>MTTELNQGEQFVADFRANAAALTTANAYNPEDEHDACGVGFIAAIDGKPRRSVVEKGIEALKAVWHRGAVDADGKTGDGAGIHVAVPQKFFKDHVKVIGHRAPDNKLAVGQVFLPRISLDAQEACRCIVETEILAFGYYIYGWRQVPINVDIIGEKANATRPEIEQIIVGNNKGVSDEQFELDLYIIRRRIEKAVKGEQINDFYICSLSARSIIYKGMFLAEQLTTFYPDLLDERFESDFAIYHQRYSTNTFPTWPLAQPFRMLAHNGEINTVKGNVNWMKAHETRMEHPAFGTHMQDLKPVIGVGLSDSGSLDTVFEVMVRAGRTAPMVKMMLVPQALTSSQTTPDNHKALIQYCNSVMEPWDGPAALAMTDGRWVVGGMDRNGLRPMRYTITTDGLIIGGSETGMVKIDETQVIEKGRLGPGEMIAVDLQSGKLYRDRELKDHLATLKPWDKWVQNTTHLDELVKTASLKGEPSDMDKAELRRRQQAFGLTMEDMELILHPMVEDGKEAIGSMGDDSPIAVLSDKYRGLHHFFRQNFSQVTNPPIDSLRERRVMSLKTRLGNLGNILDEDETQTRLLQLESPVLTTAEFRAMRDYMGDTAAEIDATFPVDGGPEALRDALRRIRQETEDAVRGGATHVILTDEAMGPARAAIPAILATGAVHTHLIRSNLRTFTSLNVRTAEGLDTHYFAVLIGVGATTVNAYLAQEAIAERHRRGLFGSMPLEKGMANYKKAIDDGLLKIMSKMGISVISSYRGGGNFEAIGLSRALVAEHFPAMVSRISGIGLNGIQKKVLEQHATAYNEEVVALPVGGFYRFRKSGDRHGWEGGVIHTLQQAVTNDSYTTFKKYSEQVNKRPPMQLRDLLELRSTKAPVPVDEVESITAIRKRFITPGMSMGALSPEAHGTLNVAMNRIGAKSDSGEGGEDPARFRPDKNGDNWNSAIKQVASGRFGVTAEYLNQCRELEIKVAQGAKPGEGGQLPGFKVTEMIARLRHSTPGVMLISPPPHHDIYSIEDLAQLIYDLKQINPDAKVTVKLVSRSGIGTIAAGVAKANADIILISGNSGGTGASPQTSIKFAGLPWEMGLSEVHQVLTLNRLRHRVRLRTDGGLKTGRDIVIAAMLGAEEFGIGTASLIAMGCIMVRQCHSNTCPVGVCVQDDKLRQKFVGTPEKVVNLFTFLAEEVREILAGLGFRSLNEVIGRTDLLHQVSRGAEHLDDLDLNPRLAQVDPGENARYCTLQGRNEVPDTLDARIVADARPLFEEGEKMQLAYNARNTQRAIGTRLSSMVTRKFGMFGLQPGHITIRLRGTAGQSLGAFAVQGIKLEVMGDANDYVGKGLSGGTIVVRPTTSSPLETNKNTIIGNTVLYGATAGKLFAAGQAGERFAVRNSGATVVVEGCGSNGCEYMTGGTAVILGRVGDNFAAGMTGGMAYVYDLDDSLPLYINDESVIFQRIEVGHYESQLKHLIEEHVTETQSRFAAEILNDWAREVTKFWQVVPKEMLNRLEVPVHLPKAISAE[6x];>[6x]MANQRMLGFVHTAQRMPDKRPAAERRQDFAEIYARFSDERANEQANRCSQCGVPFCQVHCPVSNNIPDWLKLTSEGRLEEAYEVSQATNNFPEICGRICPQDRLCEGNCVIEQSTHGAVTIGSVEKYINDTAWDQGWVKPRTPSRELGLSVGVIGAGPAGLAAAEELRAKGYEVHVYDRYDRMGGLLVYGIPGFKLEKSVVERRVKLLADAGVIYHPNFEVGRDASLPELRRKHVAVLVATGVYKARD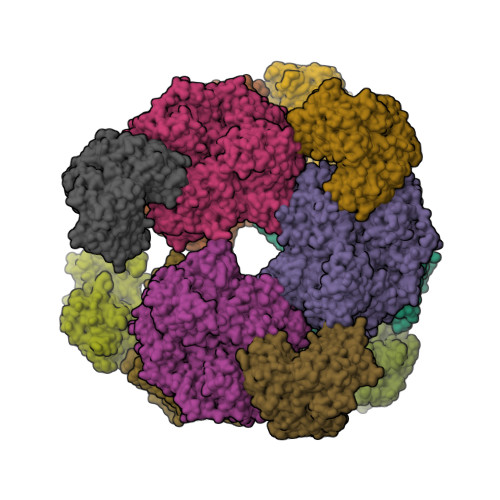IKAPGSGLGNIVAALDYLTTSNKVSLGDTVEAYENGSLNAAGKHVVVLGGGDTAMDCVRTAIRQGATSVKCLYRRDRKNMPGSQREVAHAEEEGVEFIWQAAPEGFTGDTVVTGVRAVRIHLGVADATGRQTPQVIEGSEFTVQADLVIKALGFEPEDLPNAFDEPELKVTRWGTLLVDHRTKMTNMDGVFAAGDIVRGASLVVWAIRDGRDAAEGIHAYAKAKAEAPVAVAAE>[2x]GEFMVSIMLLKVEDLHVYRGNREILKGVNLTVEENEIHAIIGPNGAGKSTLAYTIMGISGYKPTKGRIIFKGVDIIDKNITERARMGMTLAWQEPARFEGIKVKNYLMLGMNEKYKKDKEIAEEKIREALKLVNLDPDKYLDRYVDETLSGGERKRIELASIICMEPDLAILDEPDSGIDIVSFDEIKRVFDYLKDKGCSLLVITHREELAEHADRVSLICAGEVIKSGDPKEVGEFYKKECGKCYKKVPDGK;>[2x]GEFELMSIKEELMEIIEAIKYTSEKPEEIVHGKGPRIIVKESRIIDVQGDEGIILEGKEEDGKIKAKIIVKKGYKFKYPIHMCFGITEENISQIIDVEIILEEDSSISLMSHCSFPKGKGIKHIMNGIIKIGKNAKFSYNEFHYHGMDGDILVKPTVKVEIDEGGIYISNFTLTKGRIGTLDIEQEIIAKKDAIIDITTRTYAIKEDVVKVNEVVKLNGENAKCIIKSRGAAMDNSKISLKLKIEGNAPYSKGHIDCAEIVKGNAEVESIPIVVVRDDKARITHEAAIGSVDKKQLETLMAKGLDEDEATEIIVKGMIGDL

The present study focuses on the ancestor SMS from the hyperthermophilic archaeon Methanocaldococcus jannaschii. Biochemical and structural studies showed that SMS is made of a SmsC2B2 heterotetratmer wherein the SmsC subunit hosts both ATP and [Fe-S] cluster binding sites. With respect to the six components of the SUF system, SMS has only two components, SmsC and SmsB, encoded by the smsCB operon. The SmsC subunit, consisting of a RecA-like domain and a helical domain, contains all the structural motifs of the nucleotide-binding (NBD) subunits of the ABC ATPases (i.e., Walker A, Walker B, ABC signature, D-, Q-, and H-loops).

For the [Fe-S] cluster-bound structure, we chemically reconstituted the protein complex and performed crystallization inside the anoxic chamber yielding new crystal forms. Unfortunately, colorless crystals and further iron quantitation showed that the crystallized SmsC2B2 complex had no bound [Fe-S] cluster, but a sulfate anion bound to SmsC. The structure derived from crystals grown in anoxic conditions showed that the nucleotide has been displaced from the ATPase active site by a sulfate anion located into the usual site for the γ-phosphate of ATP. SmsB and SmsC assembled into a symmetric hetero-tetramer consisting of two subunits of each protein related by a 2-fold symmetry. The first N-terminal 32 residues of SmsB are disordered and were not included in the final model. However, we observed a weak extra electron density in the different maps, consistent with an α-helix likely belonging to this N-terminal region close to the center of the complex. Upon dissociation of the cluster, the C-terminal extension of SmsC unfolds, destabilizing the asymmetric SmsC-SmsC dimer observed in the cryo-EM structure, and allowing the SmsC2B2 complex to open up to adopt a conformation like the one observed in the crystal structure (intermediate 2).>[2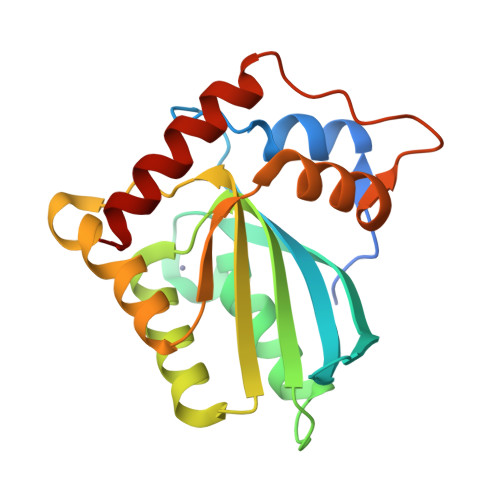x]GPGGSGGMNPQIRNPMERMDRDTFYDNFENEPILSGRSYTWLCYEVKIKRGRSNLLWDTGVFRGQVYFKPQYHAEMCFLSWFCGNQLPADKCFQITWFVSWTPCPDCVAKLAEFLSEHPNVTLTISAARLYYYSERDYRRALCRLSQAGARVKIMDYEEFAYCWENFVDNEGQQFMPWYKFDENYAFLHRTLKEILRH> MTDTATTPQTTDAPAFPSNRSCPYQLPDGYAQLRDTPGPLHRVTLYDGRQAWVVTKHEAARKLLGDPRLSSNRTDDNFPATSPRFEAVRESPQAFIGLDPPEHGTRRRMTISEFTVKRIKGMRPEVEEVVHGFLDEMLAAGPTADLVSQFALPVPSMVICRLLGVPYADHEFFQDASKRLVQSTDAQSALTARNDLAGYLDGLITQFQTEPGAGLVGALVADQLANGEIDREELISTAMLLLIAGHETTASMTSLSVIT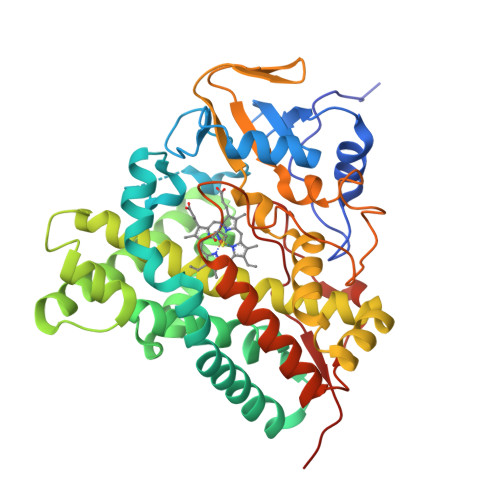LLDHPEQYAALRADRSLVPGAVEELLRYLAIADIAGGRVATADIEVEGQLIRAGEGVIVVNSIANRDGTVYEDPDALDIHRSARHHLAFGFGVHQCLGQNLARLELEVILNALMDRVPTLRLAVPVEQLVLRPGTTIQGVNELPVTWHHHHHH3-quinolin-6-ylbenzoic acid | C16 H11 N O2 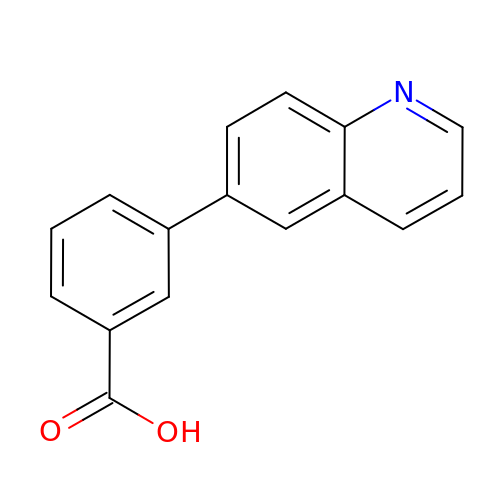| NVUDTXCAUAPCDL-UHFFFAOYSA-N>ADKELKFLVVDDFSTMRRIVRNLLKELGFNNVEEAEDGVDALNKLQAGGYGFVISDWNMPNMDGLELLKTIRADGAMSALPVLMVTAEAKKENIIAAAQAGASGYVVKPFTAATLEEKLNKIFEKLGM[3x];>MGDSILSQAEIDALLN[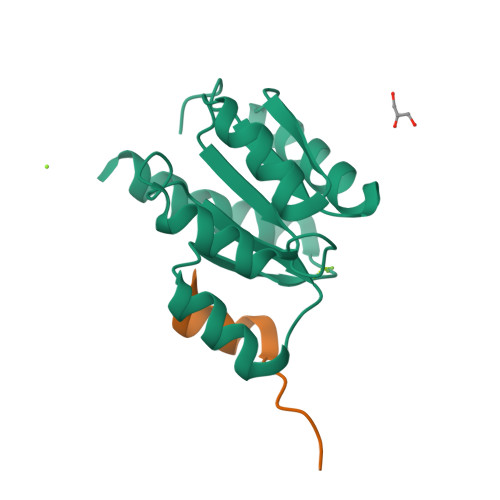3x]>MALLAEHLLKPLPADKQIETGPFLEAVSHLPPFFDCLGSPVFTPIKADISGNITKIKAVYDTNPAKFRTLQNILEVEKEMYGAEWPKVGATLALMWLKRGLRFIQVFLQSICDGERDENHPNLIRVNATKAYEMALKKYHGWIVQKIFQAALYAAPYKSDFLKALS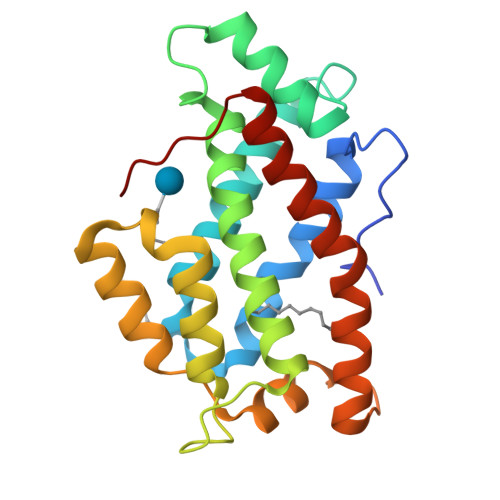KGQNVTEEECLEKIRLFLVNYTATIDVIYEMYTQMNAELNYKV[2x]AlkB family of 2-oxoglutarate (2OG or α-KG)-dependent oxygenases are evolutionarily conserved and implicated in nucleotide demethylation. Mouse ALKBH1 protein has 389 residues and consists of an N-terminal extension (NTE), a nucleotide-recognition lid (NRL), and a C-terminal double-stranded β helix (DSBH) domain. By establishing a reliable in vitro enzymatic assay, we demonstrated that ALKBH1 prefers bubbled and bulged DNAs, instead of ssDNA or dsDNA substrates. Structural studies of ALKBH1 in substrate-free and a 21-mer bulge DNA-bound state revealed the molecular determinants underlying the observed substrate preference, including unique features of a stretch-out Flip1 motif and a functionally indispensable N-terminal “α1” helix.

To obtain a stable and homogenous complex sample for crystallization, we adopted a disulfide cross-linking strategy by introducing a cysteine residue (S235C) in the catalytic pocket and a disulfide-modified cytosine within the bulge. The overall structure of DNA-bound and the free state ALKBH1 superimposed well (r.m.s.dCα = 0.555 Å), except for conformational adjustments of several flexible loops of Flip2 and Flip1 regions. As expected, the structurally stabilized Flip1 element remains in a “stretch-out” conformation even in the presence of DNA substrate, lending further supports to the lack of autonomous base-flipping capability of ALKBH1. Consistent with our previous analysis, the 21-mer bulged DNA substrate is docked onto a wide and positively charged concave surface in between Flip1, Flip2 and α1 (left). The bulged DNA adopts a B-form structure with both strands contributing to enzyme-substrate recognition primarily through “basic-backbone” interactions. Notably, two arginine residues (R24 of α1 and R159 of Flip1) insert into DNA minor grooves from both ends and function as two fingers to hold the DNA substrate (right). Such a recognition mode likely helps to orientate the DNA substrate for proper insertion of the flipped base into the active pocket, which is supported by dramatic activity loss of the R24A and R159A mutants. The observed interaction mode between ALKBH1 and bulged DNA underscores the need of both the flanking duplex/stem region and the flipped base for recognition and catalysis. Our co-crystal structural studies demonstrated that the stretch-out conformation of a K/R-rich Flip1 creates a wide and basic concave surface best for duplex DNA engagement with the flipped methyl base inserted into the active center.

> EDAFRKLFRFYRQSRPGTADLGAVIDFSEAHLARSPKPGVPQVVRFPLNVSSVTERDAERVGLEPVSKWRAYGLEGYPGFIFIPNPFLPGCQRHWVKQCLKLYSQKPNVSNLDKHMTKEETQGLWEQSKEVLRSKEVTKRRPRSLLERLRWVTLGYHYNWDSKKYSADHYTPFPSDLAFLSEQVATACGFQGFQAEAGILNYYRLDSTLGIHVDRCELDHSKPLLSFSFGQSAIFLLGGLKRDEAPTAMFMHSGDIMVMSGFSRLLNHAVPRVLPHPDGESLPHSLETPLPAVLPSNSLVEPSSVEDWQVCATYLRTARVNMTVRQVLATGQDFPL> GGSSVGRSRSPPPSRERSVRSIEQELEQLRDVTPINQWKRKRSLWDIKPPGY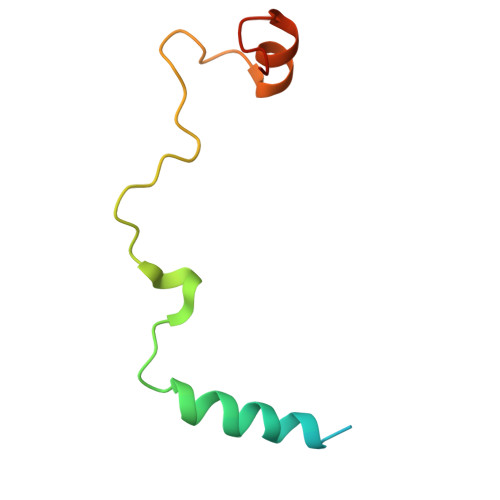ELVTADQAKMSGVFPLPGA>EQKTRPFTLPNLPLSSLSNSRAPLPISSIGISPDNVQSVQFQNGRCTLDGRLVGTTPVSLSHVAKIRGTSNGTVINLTELDGTPFHPFEGPAPIGFPDLGGCDWHINMTQFGHSSQTQYDVDTTPDTFVPHLGSIQANGIGSGNYVGVLSWISPPSHPSGSQVDLWKIPNYGSSITEATHLAPSVYPPGFGEVLVFFMSKMPGPGAYNLPCLLPQEYISHLASEQAPTVGEAALLHYVDPDTGRNLGEFKAYPDGFLTC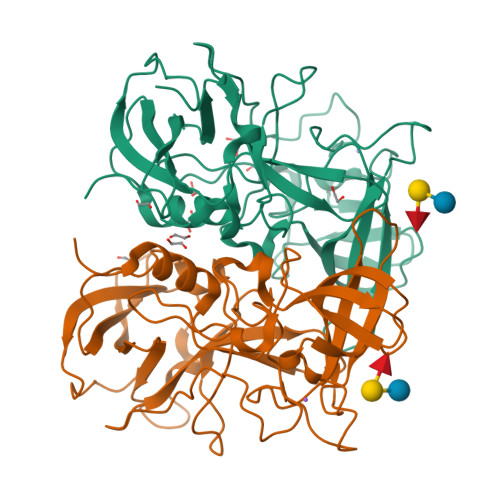VPNGASSGPQQLPINGVFVFVSWVSRFYQLKPVGTA[2x]> 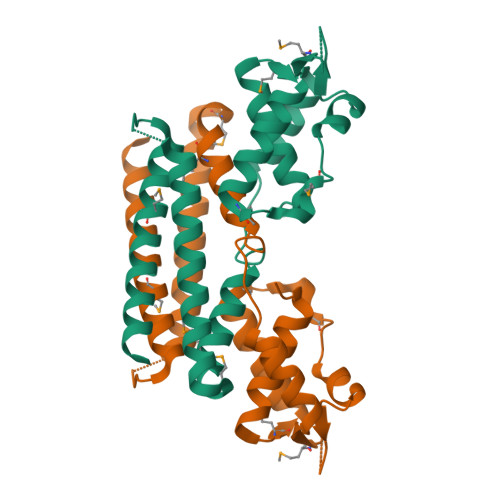GMFADNTLTPKEAVRLCALGTIASQPMRYSELAGSVRHFTSRIMGPSLELMGISIELLRYEGLVEAVDDGQGMEDDAMLAISAAGRRELHSLLTARLRPGSDLSKLVVALKMRFLGLMEAEERAHQIDLLIEGVDSELARLADLRGSDGEGGSALAAWLDHDMALLESRLAWLEDFRARL> EVGKSFKDRKMIEKMQEENRKDREKAAAKFREYFPNFVGEP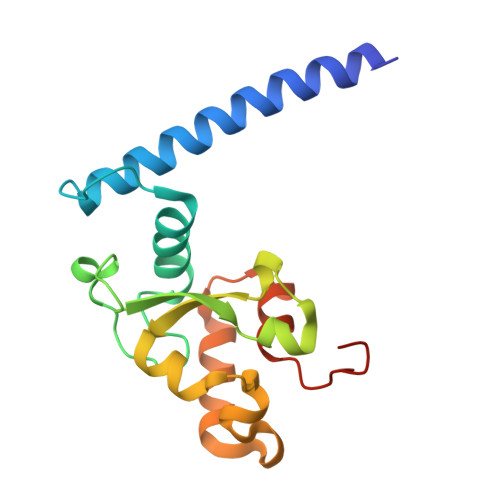KSKDILKLRLYEMQHGKCLYSGKEINLGRLNEKGYVEIDHALPFSRTWDDSFNNKVLVLGSENQNKGNQTPYEYFNGKDNSREWQEFKARVETSRFPRSKKQRILLQKFDEDGFKERNL The autonomous non-LTR retrotransposon long interspersed nuclear element-1 (LINE-1 or L1) is one the most abundant mobile elements in the human genome, comprising 17–20% of its content. ORF1p acts as a nucleic acid chaperone that binds L1 RNA, while ORF2p provides endonuclease (EN), reverse transcriptase (RT) and RNA-binding activities through three distinct functional domains. L1-EN initiates de novo L1 integration by producing a single-strand nick at a genomic site generally fitting the consensus target sequence 5′-TTTTT/AA-3′ (6,7,24,25). L1-EN belongs to the family of metal-dependent phosphohydrolases that includes apurinic/apyrimidinic endonuclease 1 (APE1) and DNase I, which are part of the exonuclease-endonuclease-phosphatase (EEP) domain superfamily.

Two mutations were introduced into L1-EN to facilitate crystallization of the enzyme complexed with DNA: D145A to prevent DNA cleavage and Y226K to alter crystal packing. The double mutant protein L1-EN-D145A/Y226K was readily crystallized in complex with two DNA substrates, dna14 and dna17, and structures were solved to a resolution of 2.8 Å. There is one DNA-protein complex in an asymmetric unit in crystals of L1-EN-D145A/Y226K with dna14 and two complexes in an asymmetric unit in crystals of the protein with dna17. Notably, the preferred scissile bond (TTTT/AA) was juxtaposed with the catalytic site in all three complexes despite differences in the lengths of the two DNA substrates and in the contacts formed between the DNA and symmetry-related molecules in the crystal lattice. The ends of the dna17 substrate interact with symmetry-related proteins, resulting in unwinding of boundary base pairs. Thus, the DNA helix is distorted at the boundaries of protein-bound dna17 but is stabilized in protein-bound dna14. Nevertheless, the conformation of the middle part of the DNA substrates containing the recognition sequence bound to the protein's active site are very similar in both dna14- and dna17-L1-EN complexes. Remarkably, the observed deviations in geometrical parameters were almost identical in all complexes of L1-EN with DNA for the middle part of the DNA substrates, particularly base pairs in positions –4 to + 4 relative to the scissile bond. In contrast, conformations of the base pairs at the ends of the DNA fragments were found to differ between different crystal forms, reflecting unique interactions with symmetry-related L1-EN molecules in the crystals. These findings suggest that conformational changes around the cleavage site are stabilized solely by interactions of the DNA with L1-EN and are not affected by crystal packing.

>MTGSNSHITILTLNINGLNSAIKRHRLASWIKSQDPSVCCIQETHLTCRDTHRLKIKGWRKIYQANGKQKKAGVAILVSDKTDFKPTKIKRDKEGHYIMVKGSIQQEELTILNIYAPNTGAPRFIKQVLSDLQRDLDSHTLIMGAFNTPLSTLDRSTRQKVNKDTQELNSALHQADLIDIYRTLHPKSTEYTFFSAPHHTYSKIDHIVGSKALLSKCKRTEIITNKLSDHSAIKLELR[2x]>[4x]MSQVTEQSVRFQTALASIKLIQASAVLDLTEDDFDFLTSNKVWIATDRSRARRCVEACVYGTLDFVGYPRFPAPVEFIAAVIAYYVHPVNIQTACLIMEGAEFTENIINGVERPVKAAELFAFTLRVRAGNTDVLTDAEENVRQKLRAEGVM;> MEQLTKNQAVATSQEAVQNQNEPQLRDENAHNDKSVHGVLNPTYQAGLRRDAVQPDIEAERKKRDEIEAGKSYCSRRFGGATCDDKSAQIYARFDKNDWRIQPAEFYRFHDAEVNTFGYF;> SNIQTGAERMPHDLSHLGFLAGQIGRLITISTTPVIAGDSFEMDAVGALRLSPLRRGLAIDSTVDIFTFYVPHRHVYGEQWIKFMKDGVNATPLPTVNTTGYIDHAAFLGTINPDTNKIPKHLFQGYLNIYNNYFKAPW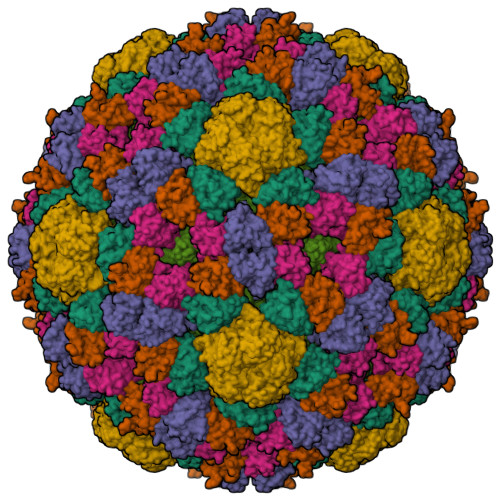MPDRTEANPNELNQDDARFGFRCCHLKNIWTAPLPPETELSRQMTTSTTSIDIMGLQAAYANLHTDQERDYFMQRYRDVISSFGGKTSYDADNRPLLVMRSNLWASGYDVDGTDQTSLGQFSGRVQQTYKHSVPRFFVPEHGTMFTLALVRFPPTATKEIQYLNAKGALTYTDIAGDPVLYGNLPPREISMKDVFRSGDSSKKFKIAEGQWYRYAPSYVSPAYHLLEGFPFIQEPPSGDLQERVLIRHHDYDQCFQSVQLLQWNSQVKFNVTVYRNLPTTRDSIMTS;> MFQTFISRHNSNFFSDKLVLTSVTPASSAPVLQTPKATSSTLYFDSLTVNAGNGGFLHCIQMDTSVNAANQVVSVGADIAFDADPKFFACLVRFESSSVPTTLPTAYDVYPLNGRHDGGYYTVKDCVTIDVLPRTPGNNVYVGFMVWSNFTATKCRGLVSLNQVIKEIICLQPLK> DGHKVGVIYIKEGQTHETEILANTMGSPDYHRFLKGLGALTRLKGATFNTQGLDRVNDMDGQYTYCWRDRVTEIVFHVTTQMPTNLEHDPQCIMKKRHIGNDFVNIVWNDSGKPFRFDTFPSQFNYVYIVITPTPRVPFLAARTARKEDDDEQRF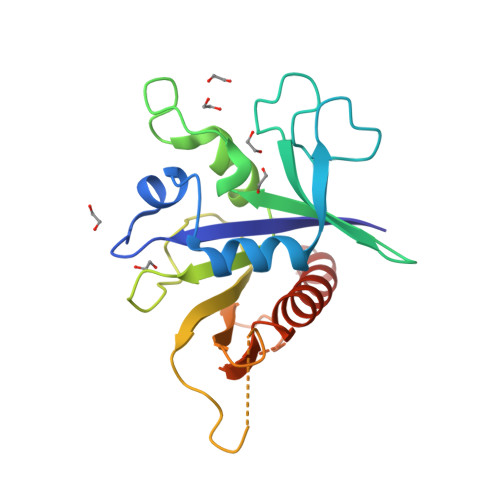VMVQVMSQPGFPEISPAAEPKIISLKALPSFVRLLALNASVFSLVWANR>QDAPEAETQAQETQGQAAARAAAADLAAGQDDEPRILEAPAPDARRVYVNDPAHFAAVTQQFVIDGEAGRVIGMIDGGFLPNPVVADDGSFIAHASTVFSRIARGERTDYVEVFDPVTLLPTADIELPDAPRFLVGTYPWMTSLTPDGKTLLFYQFSPAPAVGVVDLEGKAFKRMLDVPDCYHIFPTAPDTFFMHCRDGSLAKVAFGTEGTPEITHTEVFHPEDEFLINHPAYSQKAGRLVWPTYTGKIHQIDLSSGDAKFLPAVEALTEAERADGWRPGGWQQVAYHRALDRIYLLVDQRDEWRHKTASRFVVVLDAKTGERLAKFEMGHEIDSINVSQDEKPLLYALSTGDKTLYIHDAESGEELRSVNQL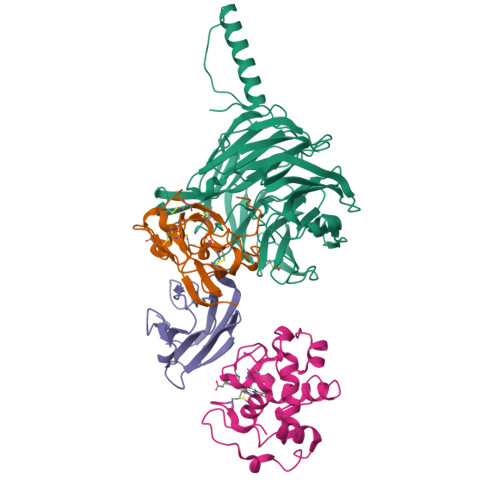GHGPQVITTADMG[4x];>[4x]ADAPAGTDPRAKWVPQDNDIQACDYWRHCSIDGNICDCSGGSLTNCPPGTKLATASWVASCYNPTDGQSYLIAYRDCCGYNVSGRCPCLNTEGELPVYRPEFANDIIWCFGAEDDAMTYHCTISPIVGKAS;>[4x]DKATIPSESPFAAAEVADGAIVVDIAKMKYETPELHVKVGDTVTWINREAMPHNVHFVAGVLGEAALKGPMMKKEQAYSLTFTEAGTYDYHCTPHPFMRGKVVVE;>APQFFNIIDGSPLNFDDAMEEGRDTEAVKHFLETGENVYNEDPEILPEAEELYAGMCSGCHGHYAEGKIGPGLNDAYWTYPGNETDVGLFSTLYGGATGQMGPMWGSLTLDEMLRTMAWVRHLYTGDPKDASWLTDEQKAGFTPFQP[4x]>TGCGCA[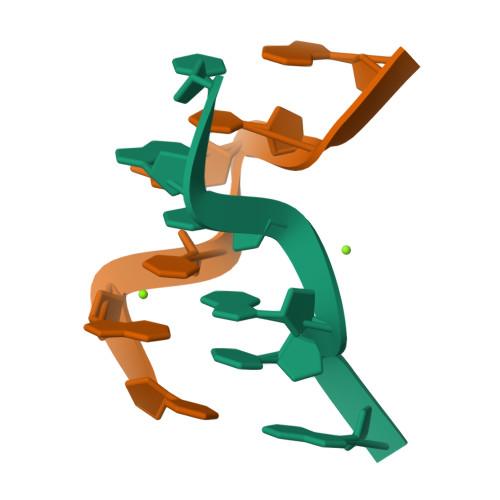2x]>GSHMTANVDGVPEKFATLGLTYDDVLLLPGASAVLPNAVDTSSRISRNVRVNIPLLSAAMDKVTESRMAISMARQGGVGVLHRNLSIEDQANQVDLVKRSESGMVANPITIHPDATLGEADALCAKFRISGVPVTDGAGKLLGIVTNRDMAFETDRSRQVREVMTPMPLVTGQVGISGVDAMELLRRHKIEKLPLVDGDGILKGLITVKDFVKAEQYPHAAKDAKGRLLVGAAVGASPEALDRAQALAEAGVDFLVVDTSHGHNSNALSWMSKIKSSVGIDVVGGNVATRDGAQALIDAGVDGIKVGVGPGSICTTRVVAGIGVPQVTAIYEASLAARAAGVPLIGDGGLQYSGDIGKALAAGADTVMLGSLLAGCEESPGELQFINGKQFKSYRGMGSLGAMQSRGQGRSYSKDRYFQAEVASDDKLVPEGIEGQVPYRGPLANVLHQLVGGLRQTMGYVGAATIEEMESKGRFVRITSAGLKESHPHDIQMTVEAPNYSRSK[16x]

IMP dehydrogenase (IMPDH) catalyzes the first step in the guanine nucleotide de novo biosynthetic pathway, at the bifurcation of the guanine and adenine routes, which share the precursor IMP. An IMPDH monomer consists of a catalytic TIM barrel (light blue) and a regulatory Bateman domain (dark blue), which is not required for catalytic activity but is essential for allosteric regulation. The basic units of IMPDH are tetramers that dimerize to form octamers upon nucleotide binding. In contrast to the eukaryotic enzymes, bacterial IMPDHs only contains two canonical allosteric binding sites in their Bateman domains.

We then set cocrystallization experiments to obtain high‐resolution structures of (p)ppGpp‐IMPDH complexes and were able to solve the structure of the IMPDH from S. coelicolor bound to ATP and ppGpp at 2.0 Å resolution (Table SS1). The AU contained 16 IMPDH monomers that are related by symmetry axes and allow the reconstruction of IMPDH octamers within the crystal lattice. These octamers are formed by dimers of tetramers assembled with a conformation that resembles, with only minor deviations, those adopted in the presence of ATP and GDP by the proteobacterial PaIMPDH enzyme. All monomers in the AU showed well‐defined electron density in the Bateman domain that could be unequivocally attributed to ATP, ppGpp, and two magnesium atoms. Surprisingly, ppGpp was bound to a previously unrecognized pocket within the Bateman domain adopting an elongated T shape conformation. 42 The (p)ppGpp binding site is different from either the second canonical (GDP2) or the third eukaryotic noncanonical site, although its δ‐ and ε‐phosphates partially occupy the canonical Site 2. The ppGpp binding pocket in StcIMPDH is mostly formed by the polar side chains of residues E118, R125, and N144, that form hydrogen bonds with different atoms of the guanine ring. The α‐ and β‐phosphates tightly interact with the basic sidechain of residues, R71, R125, K206, and K210, whereas δ‐ and ε‐phosphates, which point toward the γ‐phosphate of ATP1, coordinate two Magnesium atoms, together with the carboxylic acid of residue E188. No electron density was found in the canonical Site 2 or the noncanonical Site 3. Nonetheless, the results described above indicate that, in the presence of ATP bound to the canonical Site 1, the occupancy of the (p)ppGpp pocket is necessary and sufficient to induce the inhibited conformation.> MSITLRTYIFLDALQPQLATFIGKTARGFLPVPGQASLWVEIAPGIAINRVTDAALKATKVQPAVQVVERAYGLLEVHHFDQGEVLAAGSTILDKLEVREEGRLKPQVMTHQIIRAVEAYQTQIINRNSQGMMILPGESLFILETQPAGYAVLAANEAEKAANVHLVNVTPYGAFG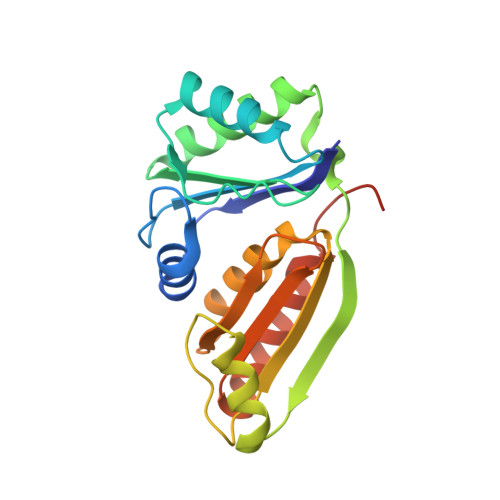RLYLAGSEAEIDAAAEAAEAAIRSVSGVAQESFRDR> NSNNKRAPYW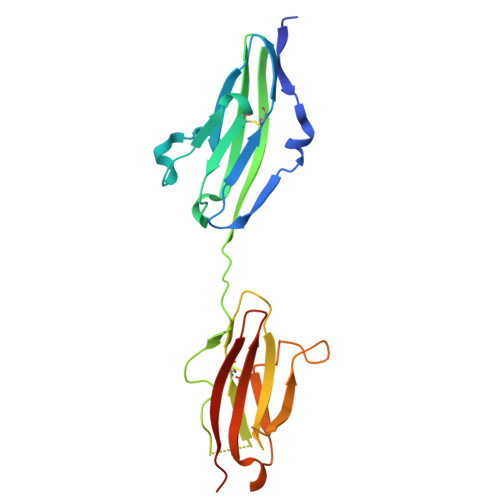TNTEKMEKRLHAVPAANTVKFRCPAGGNPMPTMRWLKNGKEFKQEHRIGGYKVRNQHWSLIMESVVPSDKGNYTCVVENEYGSINHTYHLDVVERSPHRPILQAGLPANASTVVGGDVEFVCKVYSDAQPHIQWIKHVEKNGSKYGPDGLPYLKVLKAAGVNTTDKEIEVLYIRNVTFEDAGEYTCLAGNSIGISFHSAWLTVLPAPGRE> DRSPGHHHHHHGGCPSQCSCSGTDVNCDGARFASVPAAIPITTQRLWLSNNQLTKLDPGVFDSLTQLTTLYLSNNQLTALPAGVFDKLTQLKELGLDQNQLKSIPDGAFARLPSLTHVWLHTNPWDCQCTDILYLSGWVAQHSSIVGEGWLRSWTVNPDNAKCSGTNTPVRAVTEASTSPSKCP

As antigen receptors, the lamprey utilize a family of highly diverse proteins called variable lymphocyte receptors (VLRs), which contain multiple, tandem leucine-rich repeat (LRR) motifs. The resulting VLRB protein is a 15–25 kDa, crescent-shaped protein with a continuous beta sheet where its concave surface forms the antigen binding site. Herein, we report on the characterization of a lamprey VLRB that is specific for terminal 3-O-SGal, and was isolated from a lamprey immunized with human type O erythrocytes. This VLRB, termed O6, is the first reagent to our knowledge that specifically recognizes the 3-O-SGal determinant on glycoproteins with high sensitivity. To better understand the molecular determinants of glycan recognition, we determined crystal structures of unliganded (apo) O6 and a co-crystal structure of O6 in complex with (3 S)Galβ1-4GlcNAc. This O6 VLR is relatively small compared to other characterized VLRBs, containing 178 amino acids (~19.2 kDa) and only a single LRR variable domain (LRRV1) along with the other usual LRR and CP components (LRRNT, LRR1, LRRVe, CP, and LRRCT).

The sulfate group of the ligand forms hydrogen bonds with Gln86, His109, and the backbone amide of Gly137 in an identical manner to a phosphate ion in the apo structure. Comparison of the apo and glycan complexes shows no movement of the C-terminal loop and only small changes in residue rotamers (including Trp138), indicating that the VLR is preconfigured for glycan binding (RMSD 0.28 Å for 172 aligned residues).> GGQLVMLR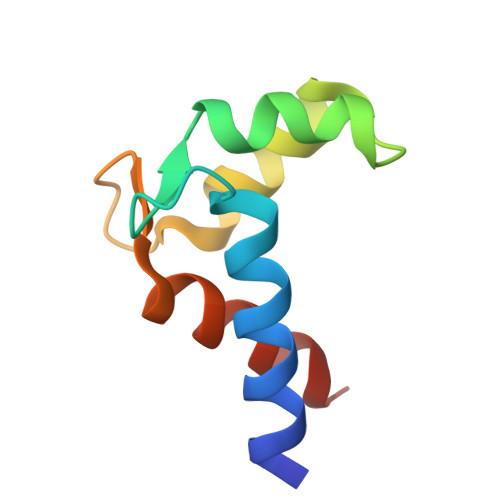KAQEFFQTCDAEGKGFIARKDMQRLHKELPLSLEELEDVFDALDADGNGYLTPQEFTTGFSHFFFSQN> AKLIGKYLMGDLLGEGSYGKVKEVLDSETLCRRAVKILKKKKLRRIPNGEANVKKEIQLLRRLRHKNVIQLVDVLYNEEKQKMYMVMEYCVCG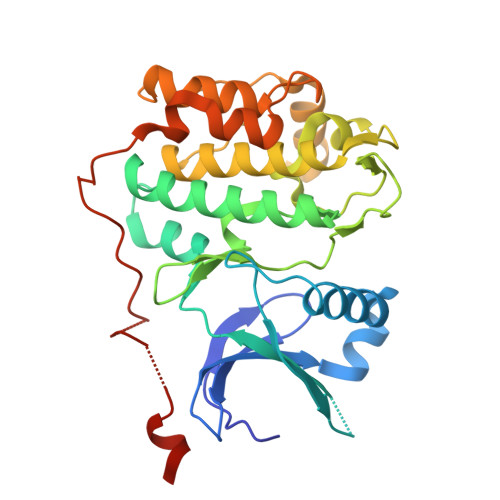MQEMLDSVPEKRFPVCQAHGYFCQLIDGLEYLHSQGIVHKDIKPGNLLLTTGGTLKISALGVAEALHPFAADDTCRTSQGSPAFQPPEIANGLDTFSGFKVDIWSAGVTLYNITTGLYPFEGDNIYKLFENIGKGSYAIPGDCGPPLSDLLKGMLEYEPAKRFSIRQIRQHSWFRKKHPPAEAPVPIPPSPDTKDRWRSMTVVPYLEDLHGA> MGHHHHHHSIVKTMIVDDSAFMRNILKRILSTTNKYVVIGEAANGADAIKMAEELQPDLISMDIVMPETDGITATKAIKE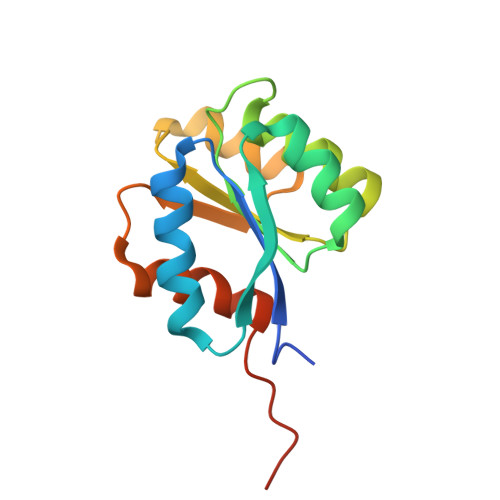KTPEIKIVMCTSVDQEQKMIDAVNAGADGYIVKPFQAPKILEQFNKLFPVLFQGPSAGLVPR> GSHMGNRRTVTLRRQPVGGLGLSIKGGSEHNVPVVISKIFEDQAADQTGMLFVGDAVLQVNGIHVENATHEEVVHLLRNAGDEVTITVEYLREAPGSAYTNFDAERDALNIETAIKTKGVDEVTIVNILTNRSNEQRQDIAFAYQRRTKKELASALKSALSGHLETVILGLLKTPAQYDASELKASMKGLGTDEDSLIEIICSRTNQELQEINRVYKEMYKTDLEKDIISDTSGDFRKLMVALAKGRRAEDG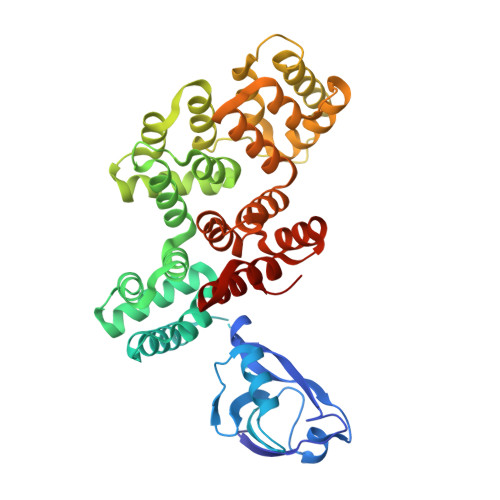SVIDYELIDQDARDLYDAGVKRKGTDVPKWISIMTERSVPHLQKVFDRYKSYSPYDMLESIRKEVKGDLENAFLNLVQCIQNKPLYFADRLYDSMKGKGTRDKVLIRIMVSRSEVDMLKIRSEFKRKYGKSLYYYIQQDTKGDYQKALLYLCGGDD(3R)-3-azanyl-4-methyl-1,3-dihydroindol-2-one | C9 H10 N2 O | 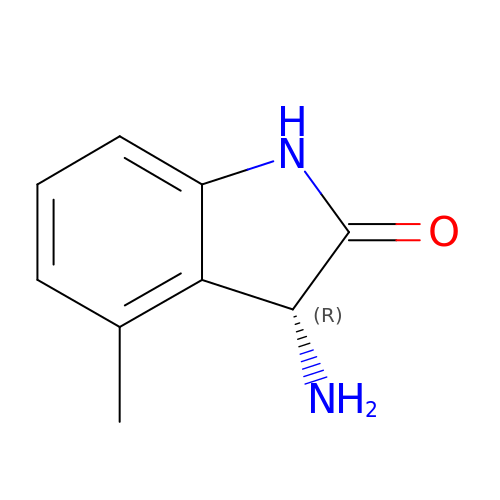DXMQUOQQGLIRSR-MRVPVSSYSA-N> MPLISSSIPNLINGVSQQPAALRLASQAEEVINCMPSPVEG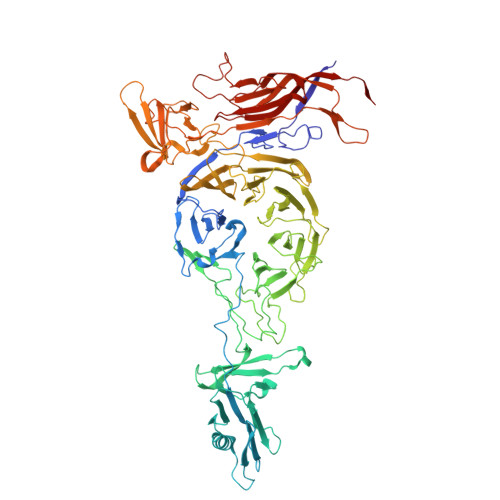LKKRPPMQHIKKLFAGSAGTGRPFTHIVDRDGVIRYLIFIQDNAIKVFDLDGNAQTVSTPNGTSYLNITGEPSSTFRVASIADFTFIVNREKTVAMDTTNKSYNWGTKSMVFIKSADFSTTYRVKLNGTEKSVTTGNSSGSAPDTVTIASDLATQLNTISGFTVTSTDYIIRITKDDGGDYTLESSDTKTADATSAIKGTVDSITDLPTIAEHNFTVRIQGSATTAFDDYFVKFEATAGSGFGPGVWRETVAPNIDHLLDKSTMPHTLVRNANGTFTFAQFNYTGRVAGDTTTAPNPTFVGSKIKNINLFRNRLVFLADENVILSAADSFERFFPETVQTLLDSDPIDISSGGTSVNFLNSSLAFANTLLLFSLHGQFRLDTGSTSVGTALTPKTATITAITTFDIVDAIDPIGVGRTVYFGIPKGDFSGLREYFLPDASGPIPLSEEVTSSVPRFVPGNLISMSPSVSEEVITMISKDQPRRVYIYKFFFDDDQKLQSSWSYWEVAANKTLLGGNVLDSDLYTCVEYSDGVYLEKTQLRPETVDSGTEFEILLDRKTTEAACSTSLINSGALGVQTVITLPYPMSGTGTMAVVGRFASNNTIAHGQVIKATAETLTGGASGNGTMTVPGDLSSAKFFVGEIYNMTYEFSTPYLKETPPGGGLAVLANPRLQLRTWSIVFDETSNFSMKITPGQRDELTYPFNGYKIGSGQFPIGTPSLATGRFRVPVMAQNIETKIVLFSDSPLPCRVQSAEWEGWYQERARRL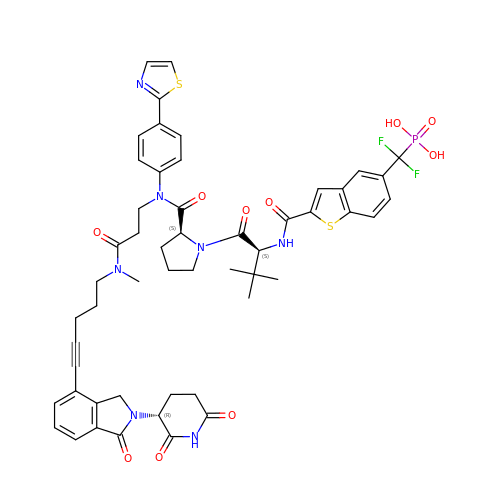N-{5-[difluoro(phosphono)methyl]-1-benzothiophene-2-carbonyl}-3-methyl-L-valyl-L-prolyl-N-(5-{2-[(3R)-2,6-dioxopiperidin-3-yl]-1-oxo-2,3-dihydro-1H-isoindol-4-yl}pent-4-yn-1-yl)-N-methyl-N~3~-[4-(1,3-thiazol-2-yl)phenyl]-beta-alaninamide | C52 H54 F2 N7 O10 P S2 | LOPYPDQOHNOVBM-JUDNIGJXSA-N>[2x]MSNKCDVVVVGGGISGMAAAKLLHDSGLNVVVLEARDRVGGRTYTLRNQKVKYVDLGGSYVGPTQNRILRLAKELGLETYKVNEVERLIHHVKGKSYPFRGPFPPVWNPITYLDHNNFWRTMDDMGREIPSDAPWKAPLAEEWDNMTMKELLDKLCWTESAKQLATLFVNLCVTAETHEVSALWFLWYVKQCGGTTRIISTTNGGQERKFVGGSGQVSERIMDLLGDRVKLERPVIYIDQTRENVLVETLNHEMYEAKYVISAIPPTLGMKIHFNPPLPMMRNQMITRVPLGSVIKCIVYYKEPFWRKKDYCGTMIIDGEEAPVAYTLDDTKPEGNYAAIMGFILAHKARKLARLTKEERLKKLCELYAKVLGSLEALEPVHYEEKNWCEEQYSGGCYTTYFPPGILTQYGRVLRQPVDRIYFAGTETATHWSGYMEGAVEAGERAAREILHAMGKIPEDEIWQSEPESVDVPAQPITTTFLERHLPSVPGLLRLIGLTTIFSATALGFLAHKRGLLVRV

The synergistic inhibition of monoamine oxidase B (MAO B) and acetylcholinesterase (AChE) is believed to provide a potentiated effect in the treatment of Alzheimer’s disease. AChE regulates cholinergic transmission at the synaptic levels by hydrolyzing the neurotransmitter acetylcholine (ACh). Monoamine oxidases A and B (MAO A and B) are enzymes cleaving the Cα–N bond of several arylalkylamines (including xenobiotics and neurotransmitters such as dopamine) upon a FAD-dependent oxidative deamination reaction. However, few X-ray structures described the binding mode of multimodal compounds targeting MAO B (covalently) or AChE (reversibly), whereas to our knowledge this is the first study reporting the binding poses of two dual reversible coumarin-based AChE-MAO B inhibitors (1 and 2)20,21 on the crystal structures of both enzymes.

Among previously reported micromolar or sub-micromolar coumarin-bearing dual inhibitors, compound 1 returned a tight-binding inhibition of MAO B (Ki = 4.5 μM) and a +5.5 °C increase in the enzyme Tm value. Indeed, a linear increase of IC50 values was observed indicating that 1 is a competitive tight-binding inhibitor of MAO B. An analogous experiment carried out with (±)-2 revealed that IC50 values are not significantly influenced by enzyme concentration, suggesting that this compound is a purely competitive inhibitor (data not shown). Therefore, all ligands had a stabilizing effect by increasing the enzyme Tm but 1 determined a remarkable +5.5 °C shift, which was in agreement with its tight-binding inhibition mechanism. In the structure of MAO B in complex with 1, the hydroxymethyl substituent at C4 lies between the Tyr398-Tyr435 pair forming the “aromatic sandwich” found in other flavin-dependent amine oxidases. The bis-N-benzylamine moiety is wedged into a pocket of the entrance cavity adopting a hook conformation that was never observed in other MAO B structures. This binding mode induce significant structural adjustments of the residues lining this portion of the active site. Phe103 and Trp119, which belong to the surface loop giving access to the enzyme cavity, are displaced by the terminal aromatic ring of 1, and, in turn, the side chains of His115 and Leu164 adopt a different conformation. As a result, the shape of the cavity, whose plasticity has been so far limited to the open/closed switch of Ile199 leading to the bipartite architecture of the MAO B active site, is in this case conserved in proximity of the flavin but significantly transformed nearby the protein surface. In MAO B, the coumarin moiety and the linker of 1 are forced to stay longitudinal by the rigid enzyme cavity and the terminal aromatic ring is accommodated in a niche of the entrance cavity rather than protruding out of the protein surface as observed with (+)-2. This unusual binding is allowed by conformational changes of the residues in the rear of the cavity (His115, Trp119, Phe103).> GHMLRHIQNSLG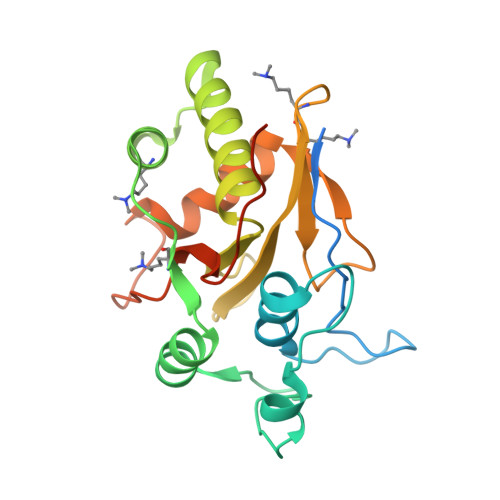SVYRSNTATPQGQIIHHRNFQSQFDTTGNTLYNNAWVCSLNVIKSRDGNNYSALEDITSDNQAFNNILEGIDIIECENLLKEMNVQKIPESSLFTNIKEALQAEVFNSTVEDDFESFISYELQNHGPLMLIRPSLGSECLHAECIVGYDSEVKKVLIYDSMNTSPEWQSNIDVYDKLTLAFNDKYKNEDCSICGLYYDGVYEPKPLHSSSWKDWCTIL> MAMRQCAIYGKGGIGKSTTTQNLVAALAEMGKKVMIVGCDPKADSTRLILHSKAQNTIMEMAAEAGTVEDLELEDVLKAGYGGVKCVESGGPEPGVGCAGRGVITAINFLEEEGAYEDDLDFVFYDVGDVVCGGFAMPIRENKAQEIYIVCSGEMMAMYAANNISKGIVKYANSGSVRLGGLICNSRNTDREDELIIALANKLGTQMIHFVPRDNVVQRAEIRRMTVIEYDPKAKQADEYRALARKVVDNKLLVIPNPITMD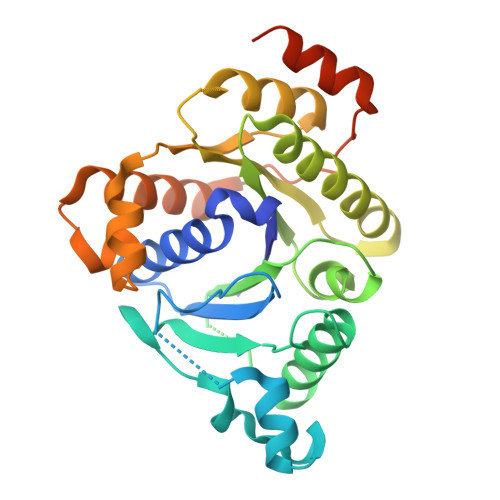ELEELLMEFGIMEVEDESIVGKTAEEV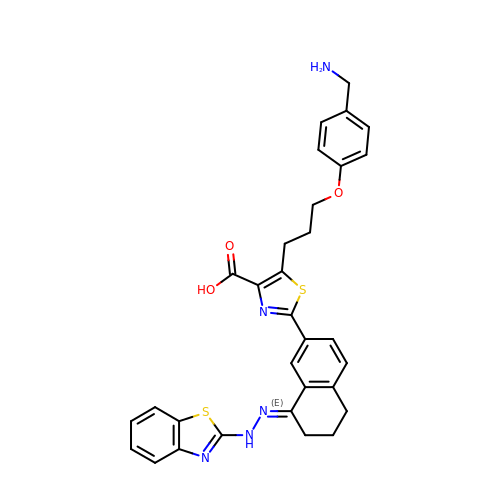5-[3-[4-(aminomethyl)phenoxy]propyl]-2-[(8E)-8-(1,3-benzothiazol-2-ylhydrazinylidene)-6,7-dihydro-5H-naphthalen-2-yl]-1,3-thiazole-4-carboxylic acid | C31 H29 N5 O3 S2 | JKMWZKPAXZBYEH-JWHWKPFMSA-N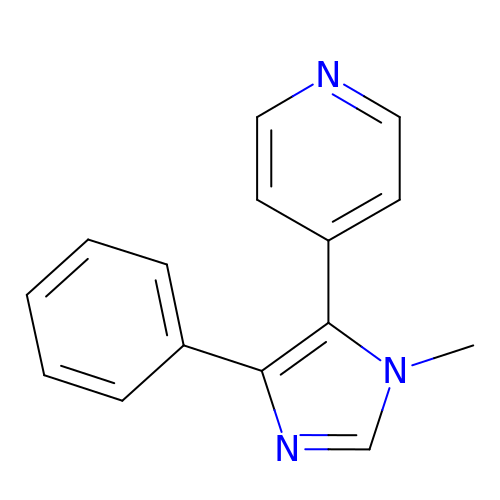4-(3-methyl-5-phenyl-imidazol-4-yl)pyridine | C15 H13 N3 | NSJCXUONRHOYTD-UHFFFAOYSA-N> MSG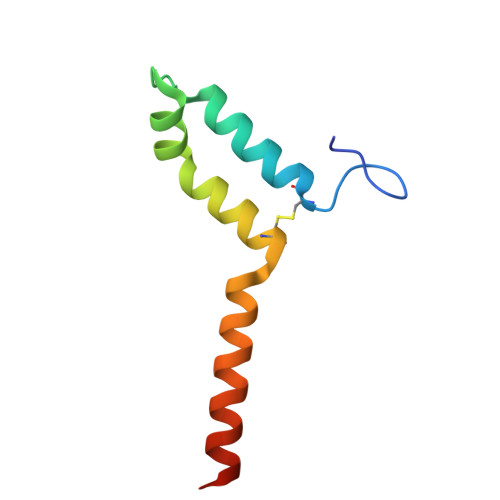FGLQSGTARCYDWYMDYLKCMDESKAPMITLRKQECSEWLEDYNECLHRDKLKLRKLLIEREKNKQEAASSS In the current study, we focused on the previously poorly characterized lipoprotein BBA14, which is known to be highly immunogenic protein recognized by sera from Lyme disease patients, but which does not have sequence similarity to any other known proteins in other organisms and is one of the 10 members of PFam143. BBA14 and another PFam143 member, BBG25, show less sequence similarity with the other PFam143 members and in contrast to the other eight PFam143 members, which are most likely cytosolic membrane proteins, BBA14 and BBG25 are lipoproteins attached to the outer membrane of B. burgdorferi. Localization studies for BBA14 and BBG25 have indicated that BBA14 is surface exposed, but BBG25 is most likely attached to the outer membrane and faces the periplasm.

Crystals of BBA14 were obtained by using the recombinant protein BBA1426–121, which corresponds to the full-length protein except the N-terminal signal peptide. The crystals were in space group P41212, with one molecule per asymmetric unit. In the obtained crystal structure, the last three C-terminal residues 119–121 were not modeled due to weak electron density, while at the N-terminus, also the residues Ala-Met-Gly remaining after TEV protease digestion were modeled. The fold of BBA14 is formed by two α-helices, designated αA and αB, comprising 27 and 30 residues, respectively. The α-helices are connected by a 20 amino acid loop region; thus, αA and αB are placed in parallel. Additionally, there is an N-terminal loop region comprising 15 amino acids; given that BBA14 is a lipoprotein, this loop likely serves as a flexible region that connects the folded region to the cell membrane. By comparing with the available 3D protein structures deposited in the Protein Data Bank (PDB) using PDBeFold, the crystal structure of BBA14 revealed a structural similarity with the antitoxin epsilon from the toxin-antitoxin system in Streptococcus pyogenes. BBA14 and the antitoxin epsilon from S. pyogenes showed high overall fold similarity (Cα root-mean-square deviation of 2.90 Ǻ) but only 20% amino acid sequence identity. Although there is a noticeable structural variability at the loop regions, the α-helices that in the S. pyogenes antitoxin are responsible for the interaction with the toxin are largely conserved. In addition, the predicted structure of BBA14 (all the predictions were done before the crystal structure of BBA14 was deposited in the Protein Data Bank (PDB)) corresponded very well to the crystal structure of BBA14 (Cα root-mean-square deviation of 0.63 Ǻ).

> GAMGLPEEPSSPQESTLKALSLYEAHLSSYIMYLQTFLVKTKQKVNNKNYPEFTLFDTSKLKKDQTLKSIKTNIAALKNHIDKIKPIAMQIYKKYSKNIP2-[(morpholin-4-yl)methyl]phenol | C11 H15 N O2 | 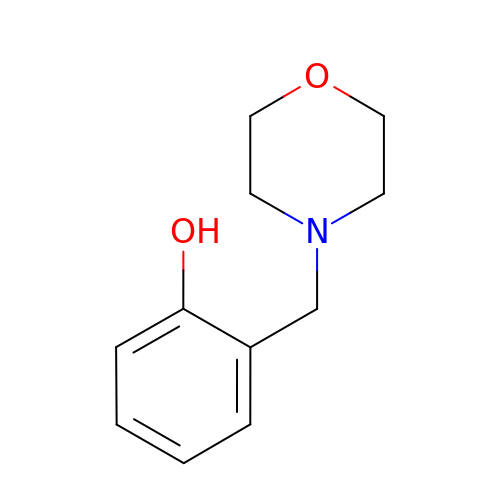OYLIEVIKIUHKTG-UHFFFAOYSA-N>[3x]MQHNLIAFLSDVGSADEAHALCKGVMYGVAPAATIVDITHDVAPFDVREGALFLADVPHSFPAHTVICAYVYPETGTATHTIAVRNEKGQLLVGPNNGLLSFALDASPAV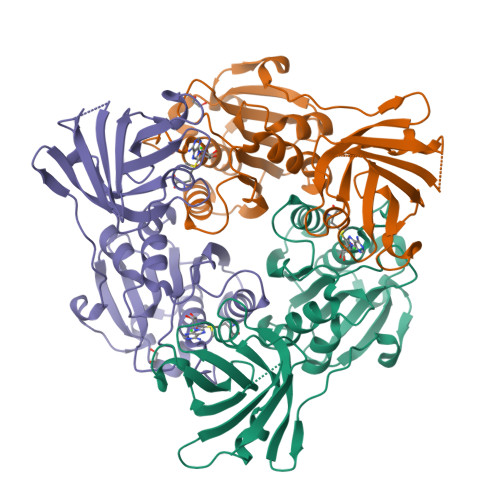ECHEVLSPDVMNQPVTPTWYGKDIVAACAAHLAAGTDLAAVGPRIDPKQIVRLPYASASEVEGGIRGEVVRIDRAFGNVWTNIPTHLIGSMLQDGERLEVKIEALSDTVLELPFCKTFGEVDEGQPLLYLNSRGRLALGLNQSNFIEKWPVVPGDSITVSPRVPDSNLGPVLG>MGAMKNCVIVSAVRTAIGSFNGSLASTSAIDLGATVIKAAIERAKIDSQHVDEVIMGNVLQAGLGQNPARQALLKSGLAETVCGFTVNKVCGSGLKSVALAAQAIQAGQAQSIVAGGMENMSLAPYLLDAKARSGYRLGDGQVYDVILRDGLMCATHGYHMGITAENVAKEYGITREMQDELALHSQRKAAAAIESGAFTAEIVPVNVVTRKKTFVFSQDEFPKANSTAEALG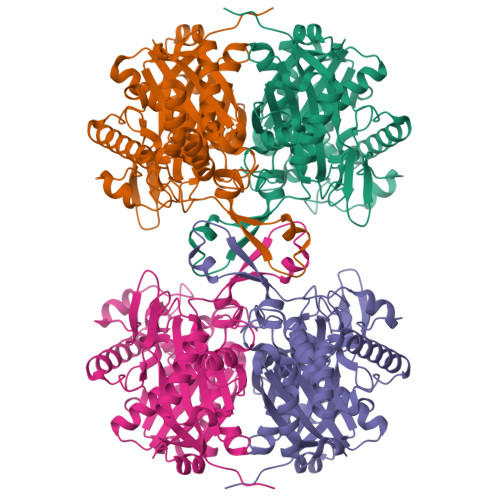ALRPAFDKAGTVTAGNASGINDGAAALVIMEESAALAAGLTPLARIKSYASGGVPPALMGMGPVPATQKALQLAGLQLADIDLIEANEAFAAQFLAVGKNLGFDSEKVNVNGGAIALGHPIGASGARILVTLLHAMQARDKTLGLATLCIGGGQGIAMVIERLNLEHHHHHH[4x]> MQKINNINNNKQMLTRKEDLLTVLKQISALKYVSNLYEFLLATEKIVQTSELDTQFQEFLTTTIIASEQNLVENYKQKYNQPNFSQLTIKQVIDDSIILLGNKQNYVQQIGTTTIGFYVEYENINLSRQTLYSSNFRNLLNIFGEEDFKYFLIDFLVFTKVEQNGYLQVAGVCLNQYFSVQVKQKKWYKNNFNMNGKATSNNNQNNANLSNEKKQENQYIYPEIQRSQIFYCNHMGREPGVFKSSFFNYSEIKKGFQFKVIQEKLQGRQFINSDKIKPDHPQTIIKKTLLKEYQSKNFSCQEERDLFLEFTEKIVQNFHNINFNYLLKKFCKLPENYQSLKSQVKQIVQSENKANQQSCENLFNSLYDTEISYKQIT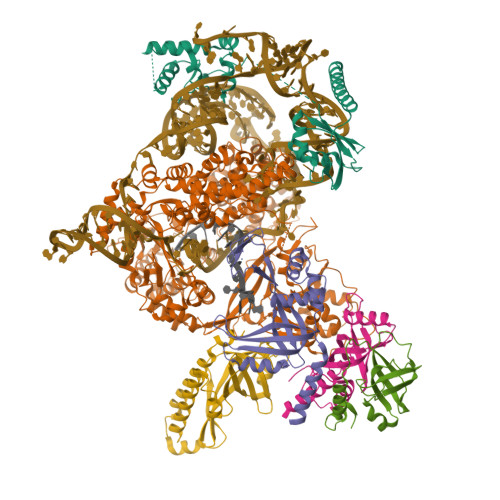NFLRQIIQNCVPNQLLGKKNFKVFLEKLYEFVQMKRFENQKVLDYICFMDVFDVEWFVDLKNQKFTQKRKYISDKRKILGDLIVFIINKIVIPVLRYNFYITEKHKEGSQIFYYRKPIWKLVSKLTIVKLEEENLEKVEEKLIPEDSFQKYPQGKLRIIPKKGSFRPIMTFLRKDKQKNIKLNLNQILMDSQLVFRNLKDMLGQKIGYSVFDNKQISEKFAQFIEKWKNKGRPQLYYVTLDIKKCYDSIDQMKLLNFFNQSDLIQDTYFINKYLLFQRNKRPLLQIQQTNNLNSAMEIEEEKINKKPFKMDNINFPYYFNLKERQIAYSLYDDDDQILQKGFKEIQSDDRPFIVINQDKPRCITKDIIHNHLKHISQYNVISFNKVKFRQKRGIPQGLNISGVLCSFYFGKLEEEYTQFLKNAEQVNGSINLLMRLTDDYLFISDSQQNALNLIVQLQNCANNNGFMFNDQKITTNFQFPQEDYNLEHFKISVQNECQWIGKSIDMNTLEIKSIQKQTQQEINQTINVAISIKNLKSQLKNKLRSLFLNQLIDYFNPNINSFEGLCRQLYHHSKATVMKFYPFMTKLFQIDLKKSKQYSVQYGKENTNENFLKDILYYTVEDVCKILCYLQFEDEINSNIKEIFKNLYSWIMWDIIVSYLKKKKQFKGYLNKLLQKIRKSRFFYLKEGCKSLQLILSQQKYQLNKKELEAIEFIDLNNLIQDIKTLIPKISAKSNQQNTN;> MKLTKGGSYILKKVDRKQFYQDEEIVMQIKKILGQKTTDCKQYIKCECIDGLGDEALIYFEMLANQNQHLQKNDVIMIQDYLNDKTQNDKIVVLVTRFQFCKASHVQPKTAQKESIQLLNTEKTIIQKSKITKNPAEEVLKFIEVNEKDNSSNSEDMIIEQQKQEIKNNQKEKQSINGFNLEDSYSNISDITNFGGKSNFNIGSLSDQLSKQTLLISQLQVGKNRFSFKFEGRVVYKSSTFQNQQDSKYFFITAQDANNQEINLSFWQKVDQSYQTLKVGQYYYFIGGEVKQFKNNLELKFKFGDYQIIPKETLSANYVQPLALQPSKQFGNDSIGDSDYSIHNLIEKEESIAQKGYNGQKNNKYRQNNNNSKHTLLISEVLKTSKQYLSVLAQVVDIQSSDKNIRLKICDNSCNQELKVVIFPDLCYEWRDKFSINKWYYFNEFVRQIYNDEVQLKNNIHSSIKESDDQRKVITYNQEQGVFKKSISINSNDSFEIKPKISYKNNSNQEQRIYSSIEEIIQQAQASEIGQKKEFYVYGNLVSIQMKNKLYYYRCTCQGKSVLKYHGDSFFCESCQQFINPQVHLMLRAFVQDSTGTIPVMIFDQQSSQLINQIDPSIHVQEAGQYVKNCIENGQEEIIRQLFSKLDFARFIFEIQFENKEFNNEQEIAYKVLKIEKENIKEESKYLLKKLEHLINNNQNN;> MSNRVQGGFDNNSGNNQSAQKQQAEKIPQITVPLNCFMINQIVKAAKENPQAHSGNHYEWYGAFENAIITAKFEFLQSINDSPKIMGKLSDSTGCIEVVIQKSKMSDELPEFVQAYEIELQNNGNRHKYVRAMLKMRKNAQIQLLYFSIVNDANEISRHGLDLCLRYLQRKHGIEDFMHMTNDKAHNNHNASAQKVHYQIDRNQQPKEQVLELMRQILKHNPNDQIPKSKIIEFFQSQLNQVQINQILQQLVSANEIFSVGSDNYLLNV;> MDAEQEQVMYPRILFEQMAQFRGKKVTVVGNVCNEDQNDSLVIEFGPTGLNQHVVIDNYRRVDLNNTTKFVEIRGVVLNQNIVSCEELTEFEQKDPFDFDTYSKLIHLSQSDKLSSLFTDQ;> MKLLLQNQNIFQKLKNTLNGCIKKFYDTYQDLEQMQKFEMIVEDKLLFRYSCSQSEMFSAQIQAHYLEKRVLQLTDGNVKYIVNFRDKGVLDKANFFDTPNNSLVIIRQWSYEIYYTKNTFQINLVIDEMRCIDIITTIFYCKLELDFTQGIKGISKSSSFSNQIYEYSAQYYKAIQLLKKLLINDSYISELYNSTKSKQQPRLFIFQSFKPKMNLAEQNLSRQFEQCQQDDFGDGCLLQIVNYTHQSLKQIENKNNSNQIVNGQNEISKKKRVLKSNEDLYKISLQKQLKIFQEEEIELHSQSTIRNQTNQQLETFESDTSKRNSEKILHSINELNTSKQKVNQMNSSQHQIQKLENNNLNKNILNQINENDIKNELEERQQQHLTQSFNSKAQLKKIITLKKNQDILLFKPQEQEGSKKY;> MDEYLENTNLEELEQECFMEDYQHEDVVEQENHQVDANDIYENQQMNDESQLNQDVKISQQKEQAVEMIEEQQQNNQDKFKQFQDCMAHITELNFKRNYQNLTEQSSSNNVVAEELDIKESLKLQMEYYFCDTNLTHDSYLRGIISKSPKNCVDIKVFLKFNKIQQILKQIQDKQIVSTYGIENQSQKKNHKNYKNQNATFSKKDLIHLIRDSLKESKILKVKMDSLKVKRRFPFNLEQALKNSKQRTLYIDFLPPKCSKQTLVSIFGNFRIININLPLQKNSQLCQGFAFIEFFSEEEANQALITKNSSIPKELILLTEKKIGQGSIRIITYKKWQEEKQSFKELSKNQNEQKNKNMNQSRKASDEFVSIDVEIKQNCLIKIINIPQGTLKAEVVLAVRHLGYEFYCDYIDENSNQINSNKISLSTQQQNTAQCSNIQIENNLIQQDQHPQLNDLLKEGQAMIRFQNSDEQRLAIQKLLNHNNNKLQIEIRGQICDVISTIPEDEEKNYWNYIKFKKNEFRKFFFMKKQQKKQNITQNYNK>MKNDLIRPNVLSVKIISNVSPEMAKKLELEPHHKSLGLITADCDDVTYTALDEATKAAEVDVVYARSMYAGAGNASTKLAGEVIGILAGPSPAEVRSGLNATLDFIDSGVGFVSANEDDSICYYAQCVSRTGSYLSKT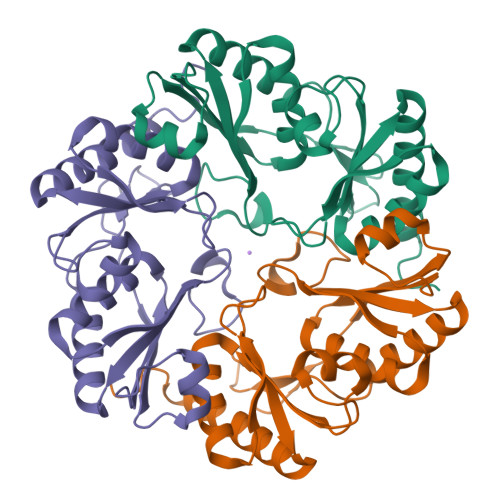AGIREGEALAYLVAPPLEAMYALDAALKAADVEMCEFFAPPTETNFAGALLTGSQSACKAACDAFAEAVQSVASNPLGFLEHHHHHH[3x]> MHHHHHHRDHRPTATDELIQASKLKQIQEHAKAILLINRQLQDILPKGLKTQVRAANVRGGNLVLEA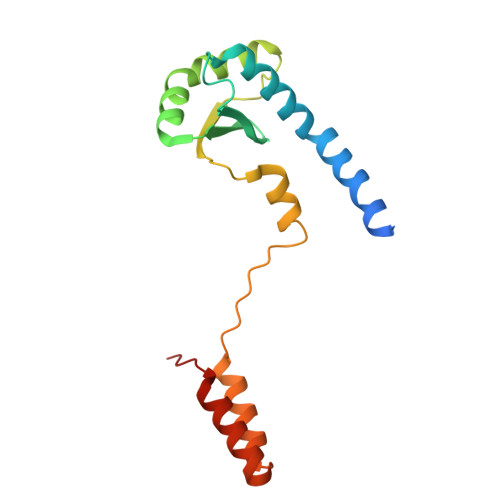ASAALKMKVDYERLHILTQLRQNGFGHLISIEVRVNPELYRQSKITSEDARAANPRPPLSEHAAHVLLAIADQASDKVKKRLQSLARLAKANQKDD(3~{R})-3-[[5-[(4,4-dimethylpiperidin-1-yl)methyl]-1~{H}-benzimidazol-2-yl]methyl]-1-[6-[(phenylmethyl)amino]pyrimidin-4-yl]piperidin-3-ol 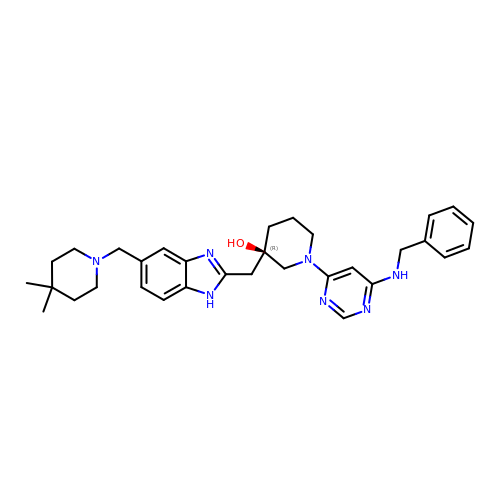| C32 H41 N7 O | YTMRIXJBQMOKPZ-JGCGQSQUSA-N> MGSSHHHHHHSQDPNSMDPLAVS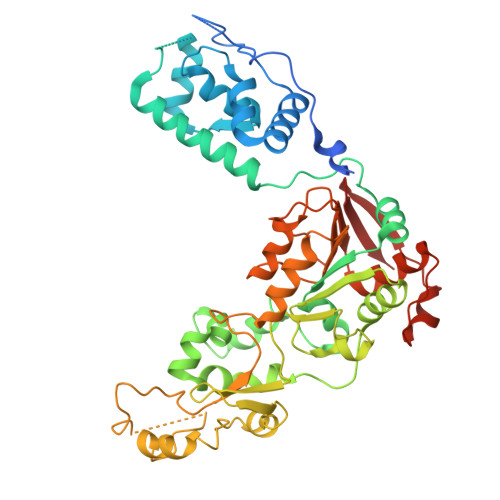AASVVSMSNDVLKPETPKGPIIISKNPSNGIFYGPSFTKRESLNARMFLKYYGAHKFLDTYLPEDLNSLYIYYLIKLLGFEVKDQALIGTINSIVHINSQERVQDLGSAISVTNVEDPLAKKQTVRLIKDLQRAINKVLCTRLRLSNFFTIDHFIQKLHTARKILVLTGAGVSTSLGIPDFRSSEGFYSKIKHLGLDDPQDVFNYNIFMHDPSVFYNIANMVLPPEKIYSPLHSFIKMLQMKGKLLRNYTQNIDNLESYAGISTDKLVQCHGSFATATCVTCHWNLPGERIFNKIRNLELPLCPYCYKKRREYFPEGYNNKVGVAASQGSMSERPPYILNSYGVLKPDITFFGEALPNKFHKSIREDILECDLLICIGTSLKVAPVSEIVNMVPSHVPQVLINRDPVKHAEFDLSLLGYCDDIAAMVAQKCGWTIPHKKWNDLKNKNFKSQEKDKGVYVVTSDEHPKTL The eukaryotic primase is a heterodimer of catalytic and regulatory subunits that is associated with the catalytic subunit of Pol α and its accessory B subunit in a constitutive heterotetrameric assembly, the Pol α/primase complex. In contrast, the Pol α/primase complex produces longer, composite RNA-DNA primers that result from the concerted enzymatic activities of primase and Pol α (Chang et al., 1984; Hu et al., 1984; Singh, et al., 1986). We have determined crystal structures of the catalytic core (349–1258; 910 amino acids) of yeast Pol α in unliganded form (apo), bound to an RNA primer/DNA template duplex (binary complex) and in a productive complex with RNA primer/DNA template and incoming dGTP (ternary complex). The catalytic region of Pol α adopts the universal ‘right-hand' DNA polymerase fold consisting of a palm domain harboring the active site, a fingers domain that interacts with the incoming nucleotide and a thumb domain that grips the primer-template duplex.

Further insight as to the possible structural basis for a termination mechanism can be obtained by comparing the structures of isolated and actively copying Pol α, which reveals a striking difference in the position of the thumb domain. In order to adopt the conformation observed in ternary complex, the thumb domain of Pol α must rotate inwards by about 20°, a large conformational rearrangement compared for instance with the limited movement of the thumb domain observed in structures of isolated and copying RB69 Pol. In comparison, the structure of the isolated polymerase displays considerable conformational fluctuations, indicative of large-scale conformational changes and local loss of secondary structure that affect in particular the N-amino terminal region and the thumb domain.

> TDTFQMFWLDYCEVNNTLILFGKVKLKDDNCVSAMVQINGLCRELFFLPREGKTPTDIHEEIIPLLMDKYGLDNIRAKPQKMKYSFELPDIPSESDYLKVLLPYQTPKSSRDTIPSDLSSDTFYHVFGGNSNIFESFVIQNRIMGPCWLDIKGADFNSIRNASHCAVEVSVDKPQNITPTTTKTMPNLRCLSLSIQTLMNPKENKQEIVSITLSAYRNISLDSPIPENIKPDDLCTLVRPPQSTSFPLGLAALAKQKLPGRVRLFNNEKAMLSCFCAMLKVEDPDVIIGHRLQNVYLDVLAHRMHDLNIPTFSSIGRRLRRTWPEKFGRGNSNMNHFFISDICSGRLICDIANEMGQSLTPKCQSWDLSEMYQVTCEKEHKPLDIDYQNPQYQNDVNSMTMALQENITNCMISAEVSYRIQLLTLTKQLTNLAGNAWAQTLGGTRAGRNEYILLHEFSRNGFIVPDKEGNRSRAQKQRQNEENADAPVNSKKAKYQGGLVFEPEKGLHKNYVLVMDFNSLYPSIIQEFNICFTTVDRNKEDIDELPSVPPSEVDQGVLPRLLANLVDRRREVKKVMKTETDPHKRVQCDIRQQALKLTANSMYGCLGYVNSRFYAKPLAMLVTNKGREILMNTRQLAESMNLLVVYGDTDSVMIDTGCDNYADAIKIGLGFKRLVNERYRLLEIDIDNVFKKLLLHAKKKYAALTVNLDKNGNGTTVLEVKGLDMKRREFCPLSRDVSIHVLNTILSDKDPEEALQEVYDYLEDIRIKVETNNIRIDKYKINMKLSKDPKAYPGGKNMPAVQVALRMRKAGRVVKAGSVITFVITKQDEIDNAADTPALSVAERAHALNEVMIKSNNLIPDPQYYLEKQIFAPVERLLERIDSFNVVRLSEALGLDSKKYFRREGGNNNG> AGSMEVIATAHGGPEVLAVRPSSHTPD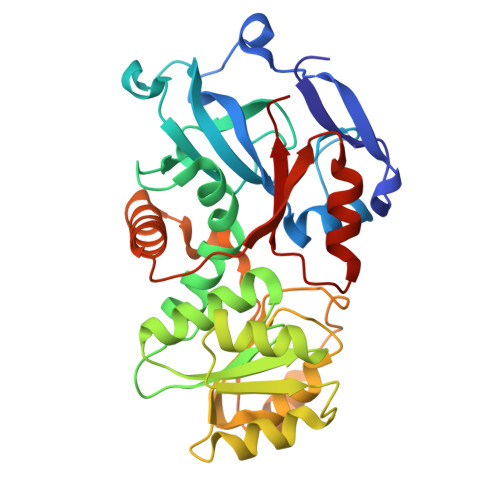ATQLEEGQVLVRNAYAGVNFIDTYFLCGLYKKPAMPYVVGEEGAGAVVKVGAGVPESMLGKRVAYFGGAGCTGSYAAFTVAPASALREVPDGVTDAEAAAVMCQGLTAHYLVDSSYPCGPGSTVVVHAAAGGTGLLVCQMAKLRGARVIGICGGAEKATLARSVGRADVVIDYVATPDWAPLARAAAPQGVDAVYDGVGQATFAGSLSVLRPRGYMITFGNASGAVPPVSPLELSRAGSVYLQRPTLGNFMRTPEEAQRRTSEVFGWVASKQVQLTIGREYPLHEAAQALTDLQSRKTTGKLLLKCIDD>[2x]MIGRRPQGLRAAASLKKQQQLEKQKQEASYELSGNSSPSKENGSENVDNGEMEDETMLVYTEEDNISQLWGLYEMSREKLENDDIDASVSLVFGTIHEADRILRNTEDISTLPKDFHAAYSSALLAVSELFEI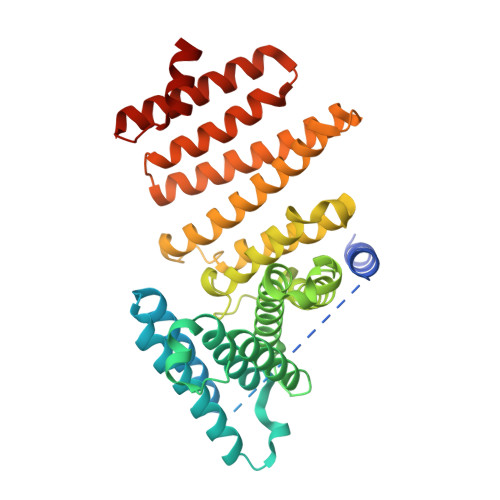AQKRLKETNTEESYIDAAIERAQLGLDAPGNESRLFLALARAYLEKVRVLVWRHDNEESLANIPVTQLVNPYIEKAIQYLRPLAQDSTEYFDALTPDSLRPLYILSSYLFQFGDQFSEAFLLDVCSIITALWLKSVVDPNTPAYYKLIAQEAVLNNYTTFAEYYMDLLDNSESNVDDLINKASSWLNNSVDTWNVIYTLDKSPERLLKLADIKMDLAQIVQDEASQDNYLKEACNAIKEAQGSGVELSPDYVEFVEAYSA>[4x]AHHHHHHMLLTDTQEQIREAARDFAQERLAPGAAARDREHAFPRAELTEMGALGFLGMLAPEEWGGSDLDMVAYALALEEIAAGDGACSTIVSVHSSVGCMPILRFGTEDQKRRFLPKMACGEWIGGFALTEPQAGSDASALKTRARLDGDHYVIDGSKQFITSGKNGNVVIVFAVTDPAAGKKGISAFIVPTDTPGYEVMSVEHKLGQHSSDTCALGFTNMRVPVENRLGAEGE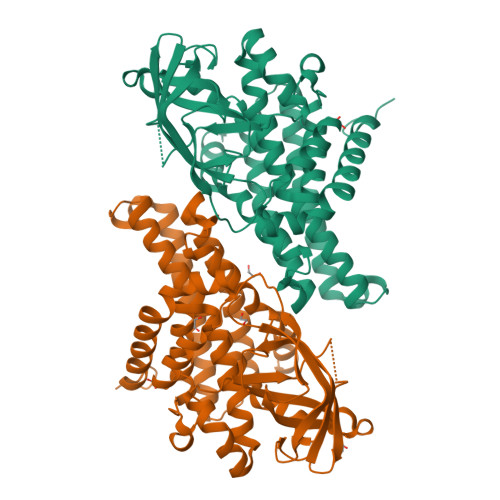GYKIALANLEGGRIGIAAQAVGMARAAFEAARDYARERITFGKPIIEHQAVAFRLADMATRIETARQMVLHAAALREAGKPCLTEASMAKLVASEMAEQVCSAAIQIHGGYGYLADYPVERIYRDVRVCQIYEGTSDVQRLVIARGL>GSREEYPDIDSEVRAILLSHAQNGITISSIKSEYRKLTGNPFPLHDNVTDFLLTIPNVTAECSESGKRIFNLKASLKNGHLLDMVLNQ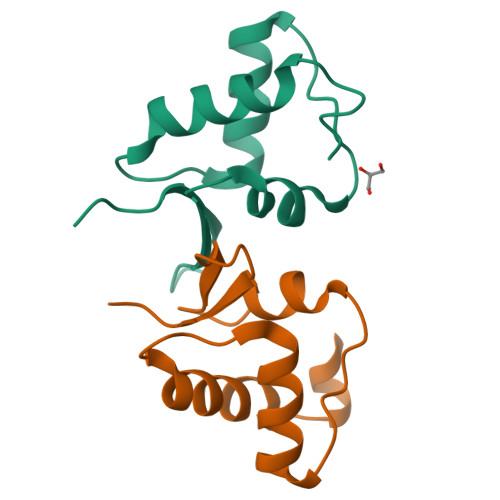KERTS[6x]> MAQFAFESDLHSLLQLDAPIPNAPPARWQRKAKEAAGPAPSPMRAANRSHSAGRTPGRTPGKSSSKVQT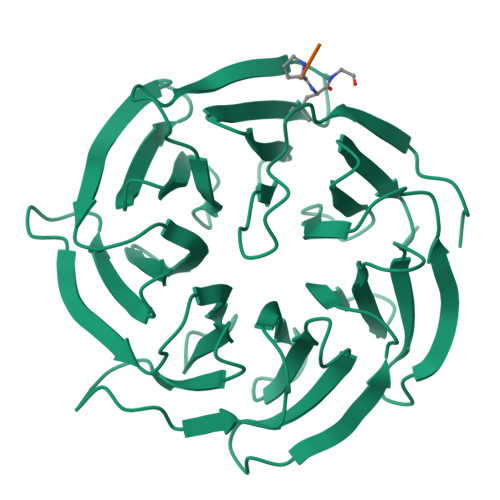TPSKPGGDRYIPHRSAAQMEVASFLLSKENQPENSQTPTKKEHQKAWALNLNGFDVEEAKILRLSGKPQNAPEGYQNRLKVLYSQKATPGSSRKTCRYIPSLPDRILDAPEIRNDYYLNLVDWSSGNVLAVALDNSVYLWSASSGDILQLLQMEQPGEYISSVAWIKEGNYLAVGTSSAEVQLWDVQQQKRLRNMTSHSARVGSLSWNSYILSSGSRSGHIHHHDVRVAEHHVATLSGHSQEVCGLRWAPDGRHLASGGNDNLVNVWPSAPGEGGWVPLQTFTQHQGAVKAVAWCPWQSNVLATGGGTSDRHIRIWNVCSGACLSAVDAHSQVCSILWSPHYKELISGHGFAQNQLVIWKYPTMAKVAELKGHTSRVLSLTMSPDGATVASAAADETLRLWRCFELDPARRREREKASAAKSSLIHQGIR;> RAPXGDISN>[3x]GSHMLSIYQDQEQRILKFLEELGEGKATT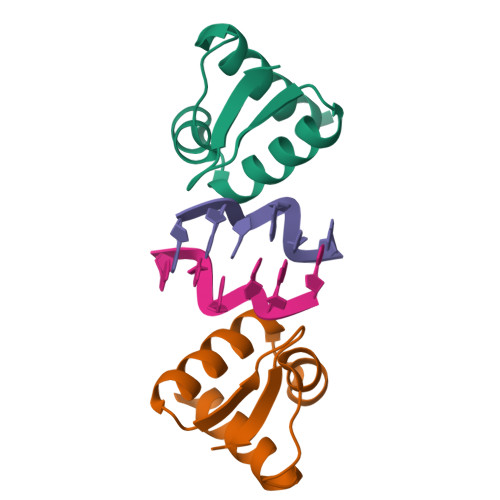AHDLSGKLGTPKKEINRVLYSLAKKGKLQKEAGTPPLWKIAVSTQAWNQHSG>MDVRLAFPLSRAEEALPRLQALGLGAEVYLDPALLEEDALFQSLRRRFSGKLSVHLPFWNLDLLSPDPEVRGLTLRRLLFGLDRAAELGADRAVFHSGIPHGRTPEEALERALPLAEALGLVVRRARTLGVRLLLENSHEPHPEAL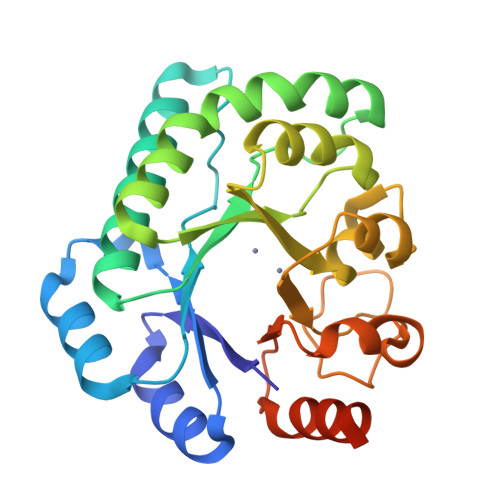RPVLEAHAGELGFCFDAAHARVFSRTPDPGPWLALAPEHLHLNDTDGVYDRHWNLGRGVLGHGAWLRPYLDRTMVLEVREDPEASLAFLQALAGEGRTALDRLLMGER[4x]>SVIKPDM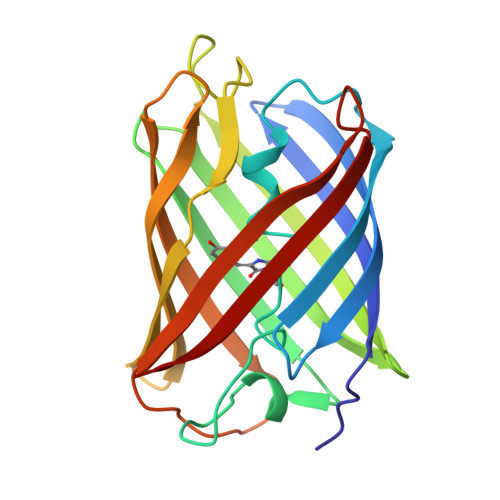KIKLRMEGAVNGHPFAIEGVGLGKPFEGKQSMDLKVKEGGPLPFAYDILTTVFCYGNRVFAKYPENIVDYFKQSFPEGYSWERSMNYEDGGICNATNDITLDGDCYIYEIRFDGVNFPANGPVMQKRTVKWEPSTEKLYVRDGVLKGDVNTALSLEGGGHYRCDFKTTYKAKKVVQLPDYHFVDHHIEIKSHDKDYSNVNLHEHAEAHS[4x]>[16x]MTATIDDQEKNQRSNPDHEEYQYLDLIRRIINVGEVRPDRTGTGTVALFAPPSFRFSLADNTLPLLTTKRVFLRGVIAELLWFVSGCTDAKMLSSQGVGIWDGNGSKEFLEKVGLGHRREGDLGPVYGFQWRHFGAEYTDADGDYKGKGVDQLQRVIDTIKNNPTDRRIILSAWNPKDLPLMALPPCHMFCQFFVSLPPADSPGSKPKLSCLMYQRSCDLGLGVPFNIASYALLTHMIALIT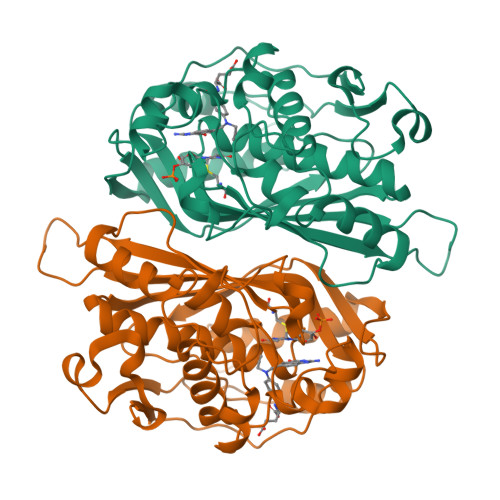DTEPHEFILQMGDAHVYRDHVEPLKTQLEREPRDFPKLKWARSKEEIGDIDGFKVEDFVVEGYKPWGKIDMKMSA>[2x]GTMSARGLNKISCSLNLQTEKLCYEDNDNDLDEELMPKHIALIMDGNRRWAKDKGLEVYEGHKHIIPKLKEICDISSKLGIQIITAFAFSTENWKRSKEEVDFLLQMFEEIYDEFSRSGVRVSIIGCKSDLPMTLQKCIALTEETTKGNKGLHLVIALNYGGYYDILQA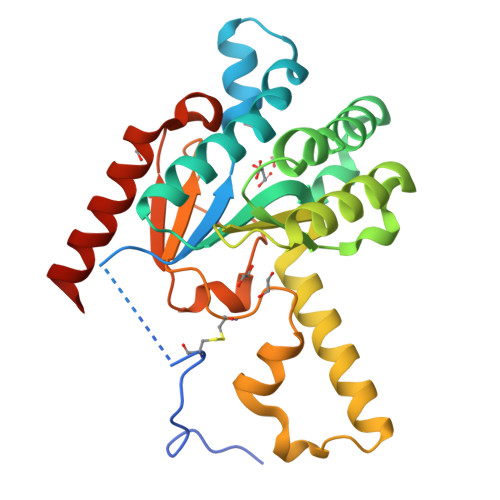TKSIVNKAMNGLLDVEDINKNLFDQELESKCPNPDLLIRTGGEQRVSNFLLWQLAYTEFYFTNTLFPDFGEEDLKEAIMNFQQRHRRFGGHTY Dr adhesins are expressed on the surface of uropathogenic and diffusely adherent strains of Escherichia coli. The major adhesin subunit (DraE/AfaE) of these organelles mediates attachment of the bacterium to the surface of the host cell and possibly intracellular invasion through its recognition of the complement regulator decay-accelerating factor (DAF) and/or members of the carcinoembryonic antigen (CEA) family. The adhesin subunit of the Dr haemagglutinin, a Dr-family member, additionally binds type IV collagen and is inhibited in all its receptor interactions by the antibiotic chloram­phenicol (CLM). In this study, previous structural work is built upon by reporting the X-ray structures of DraE bound to two chloramphenicol derivatives: chloramphenicol succinate (CLS) and bromamphenicol (BRM).

In order to establish whether substitution at the primary hydroxyl of CLM influences the binding of the small molecule to DraE, the structure of a DraE–CLS complex was determined. CLS cocrystals in space group P3 were reproducibly obtained using small-molecule concentrations between 1 and 15 mM. The aliphatic ‘tail’ and the nitro-benzene ‘head’ group were traced within this electron density. Positional and temperature (B) factor refinement confirmed that CLS was present in the binding site at full occupancy, with an average B factor of 32 Å2. No difference density was resolved for the succinate tail, implying that these atoms adopted a number of alternate conformers that were not resolved at 1.9 Å resolution. With each conformer set to an occupancy of 30%, the B factors refined to an average value of 49 Å2 for the succinate atoms, compared with an average value of 40 Å2 for the rest of the small molecule. Overall, the CLS–DraE complex structures imply that (i) substitutions at the primary hydroxyl do not significantly affect the mode of CLM binding and (ii) the nitrobenzene group is not required to bind DraE. The CLS structure in space group P3 proves that substitutions at the primary hydroxyl 3-OH do not affect the mode of CLM binding to DraE. Therefore, we hoped that increased DraE specificity could be gained from substitution at the primary hydroxyl group; unfortunately, the CLS succinate in this study did not fit the surface with a single conformation and alternative substituents to the succinyl moiety will need exploring.

>[6x]RGSHHHHHHGSFTPSGTTGTTKLTVTEKCQVRVGDLTVAKTRGQLTDAAPIGPVTVQALGCDARQVALKADTDNFEQGKFFLISDNNRDKLYVNIRPTDNSAWTTDNGVFYKNDVGSWGGIIGIYVDGQQTNTPPGNYTLTLTGGYWAK>[2x]SQKILQFEDILANTFYREHFGMYMERMDKRALI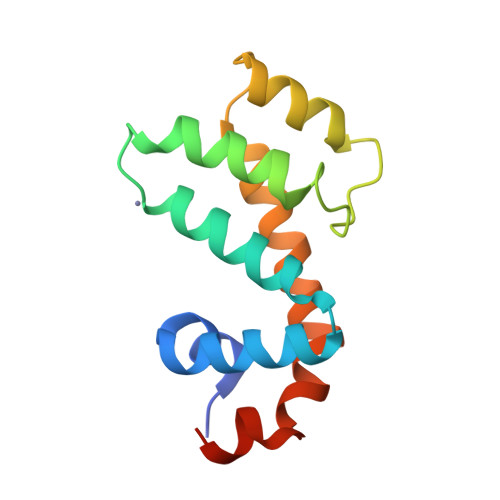SFWESVEHLKNANKNEIPQLVGEIYQNFFVESKEISVEKSLYKEIQQALVGNKGIEVFYKIQEDVYETLKDRYYPSFIVSDLYEKLLIKEE> PTHIAICLYYKLGETPLPLVIETGKDAKALQIIKLAELYDIPVIEDIPLARSLYKNIHKGQYITEDFFEPVAQ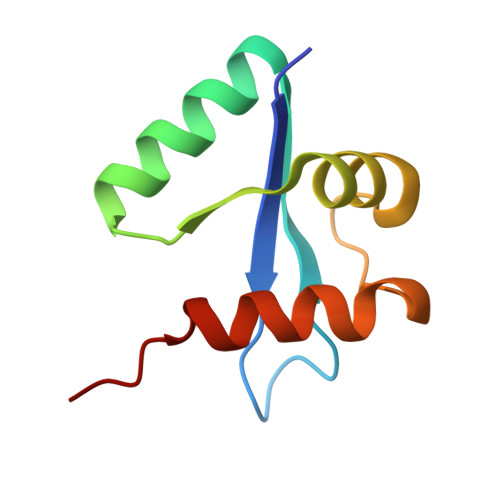LIRIAIDLDY>MILTITYTQPPATDLGYLLHKNPSRPQTFELNHGKAHIFYPEATSERCTVALLLDIDPIDLARGKKGSSGEGGLFDYVNDRPYVSSSFMSVAISRVFGTAMSGKCKEKPELAAIKLPLKAKIMMLPCKGGEEIIYRLFEPLGYKVDVEGYMLDEKFPEWGKSRYYTVSLEGEVRVR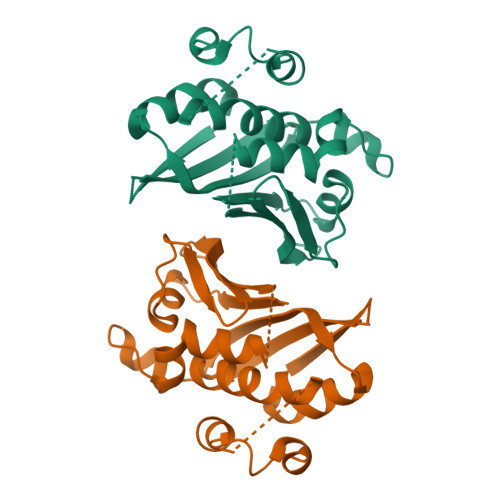DLLNHIYVLIPVLDSEKHYWVGEDEIDKLFQHGEGWLVDHPEKELITGRYLIRK[2x]>[12x]SMAQSTEQAAASAGKANTPHLTIAMITHQQPGDTFWDI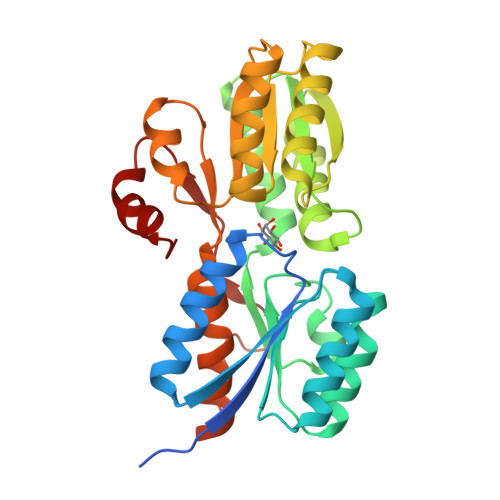IRKGALAAAAKDNVTLKYSNDPDSTKEAVLIQDAVNAKVDGIAVTIPDPPALIPAIKQAVAAGIPVVAFNAGIDQWKESGALMYFGQDETVAGQAAGARATSEGFKHVLCVLQAQGQVQLESRCNGVQQTFKGQYTKLYVNGADQPSVRTTIAAKLKQDPSIDLVITLGAPIAQLAIQAVKDAGSNAKIATFDFNTQVPAEIENGQLQWAIDQQPYVEGYEAVDSLWLYITNGDTIGGGEAVKTGPFFVDKSNVAAVAKFAERGTR> GAMASENPDVLLSRVINVVRAASSLASQDVDFYKNLDRGFSKDLKSKADKLADMANEIILSIDEHHESFELKEEDISDLWNNFGNIMDNLLEMSDHSLDKLNCAINSKSRGSDLQYLGEFSGKNFSPTKRVEKPQLKFKSPIDNSESHPFIPLLKEKPNALKPLSESLRLVDDDENNPSHYPHPYEYEIDHQEYSPEILQIREEIPSKSWDDSVPI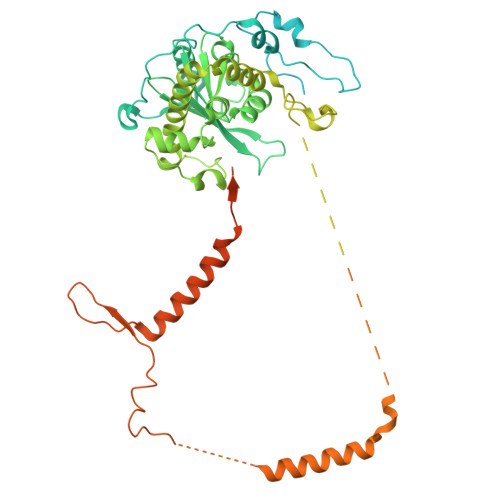WVDTSTELESMLEDLKNTKEIAVDLEHHDYRSYYGIVCLMQISTRERDYLVDTLKLRENLHILNEVFTNPSIVKVFHGAFMNIIWLQRDLGLYVVGLFDTYHASKAIGLPRHSLAYLLENFANFKTSKKYQLADWRIRPLSKPMTAYARADTHFLLNIYDQLRNKLIESNKLAGVLYESRNVAKRRFEYSKYRPLTPSSEVYSPIEKESPWKILMYQYNIPPEREVLVRELYQWRDLIARRDDESPRFVMPNQLLAALVAYTPTDVIGVVSLTNGVTEHVRQNAKLLANLIRDALRNIKNTNEEATPIPSSETKADGILLETISVPQIRDVMERFSVLCNSNISKSRAKPVTNSSILLGKILPREEHDIAYSKDGLPNKVKTEDIRIRAQNFKSALANLEDIIFEIEKPLVVPVKLEEIKTVDPASAPNHSPEIDNLDDLVVLKKKNIQKKQPAKEKGVTEKDAVDYSKIPNILSNKPG4-[(1S,2R)-2-(carboxymethyl)cyclopentane-1-carbonyl]benzoic 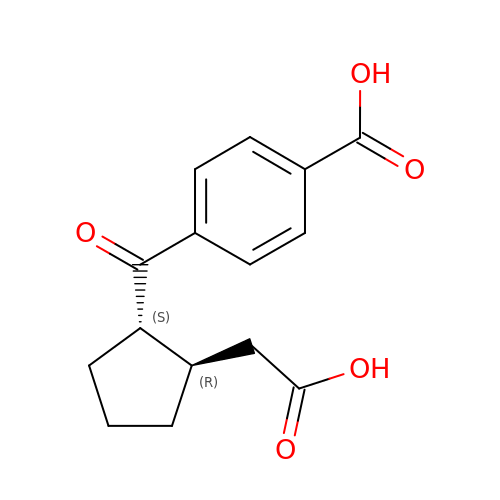acid | C15 H16 O5 | AIBKYDBZFDNIIN-NEPJUHHUSA-N>[2x]MKVEELAES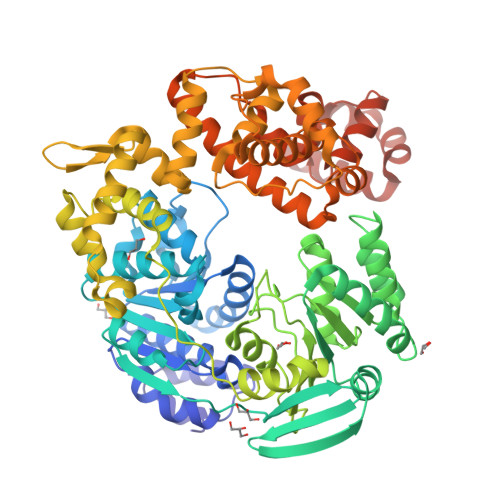ISSYAVGILKEEGIEELFPPQAEAVEKVFSGKNLLLAMPTAAGKTLLAEMAMVREAIKGGKSLYVVPLRALAGEKYESFKKWEKIGLRIGISTGDYESRDEHLGDCDIIVTTSEKADSLIRNRASWIKAVSCLVVDEIHLLDSEKRGATLEILVTKMRRMNKALRVIGLSATAPNVTEIAEWLDADYYVSDWRPVPLVEGVLCEGTLELFDGAFSTSRRVKFEELVEECVAENGGVLVFESTRRGAEKTAVKLSAITAKYVENEGLEKAILEENEGEMSRKLAECVRKGAAFHHAGLLNGQRRVVEDAFRRGNIKVVVATPTLAAGVNLPARRVIVRSPIFGGRPIKVSEYKQMAGRAGRPGMDERGEAIIIVGKRDREIAVKRYIFGEPERITSKLGVETHLRFHSLSIICDGYAKTLEELEDFFADTFFFKQNEISLSYELERVVRQLENWGMVVEDHHLAPTKLGSLVSRLYIDPLTGFIFHDVLSRMELSDIGALHLICRTPDMERLTVRKTDSWVEEEAFRLRKELSYYPSDFSVEYDWFLSEVKTALCLKDWIEEKDEDEICAKYGIAPGDLRRIVETAEWLSNAMNRIAEEVGNTSVSGLTERIKHGVKEELLELVRIRHIGRVRARKLYNAGIRNAEDIVRHREKVASLIGRGIAERVVEGISVKSLNPESAAALEHHHHHH5-chloro-4-hydroxybiphenyl-3-carboxylic acid | C13 H9 Cl O3 | 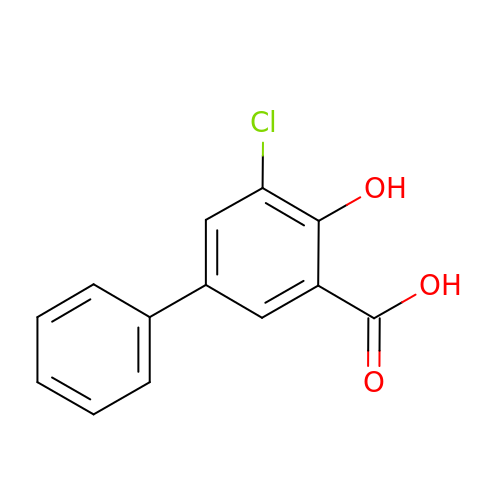RJMZIUFNDNYWDU-UHFFFAOYSA-N Sampatrilat | 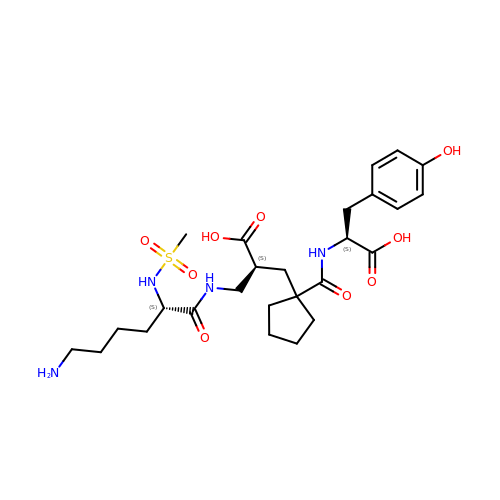C26 H40 N4 O9 S | LPUDGHQMOAHMMF-JBACZVJFSA-N> GPGYERLKEELAKAQRELKLKDEECERLSKVRDQLGQELEELTASLFEEAHKMVREANIKQA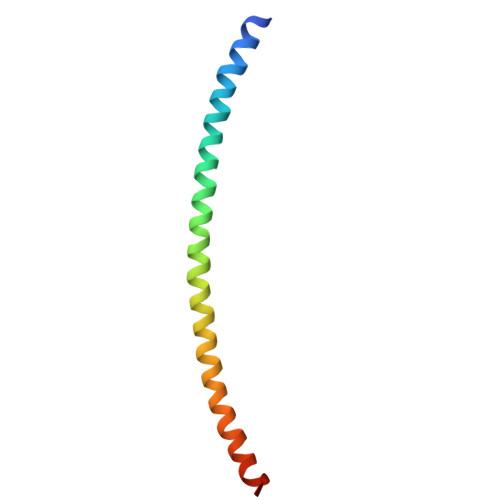TAEKQLKEAQGKIDVL>[4x]GSHMTASVPPFTVGREDPRYIELSHSDNHRFVVEPEEFFLPATPDDVVASLQKAVTEGRGVACRSGGHCGQDFVGTPRRDLVLDLHNLHAIGPAADGAGVRVGSGATVDQVQKALFRRWNAALPLGACSAVGMGGLVAG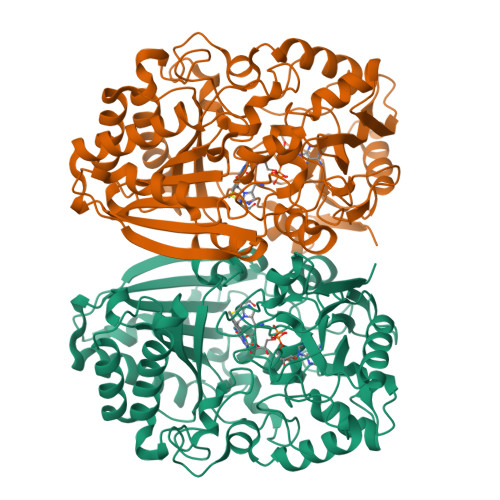GGYGPLSRQLGLVVDHLHAVEVAVVDESRTVRLVTARADDTGDLGELFWAHTGGGGGNFGVVTAYEFRSPEHLATEPVGLPRAAGRLHVQKVVFPWAMIDETSFVTVMRRFFEWHERHSEPGSPESSLFATFFVNHVSSGVLQLMVQQDADVDPEGEILARFVASLTEGTGVVGIPRGGVMSWLTGTRYMSQADCGDVMGARSASKSAYHRAAPTDEQLSVLHRHLHADHPGQASYVMFNSYGGEINRRGPSDAAVPQRDSVVKSSWFSAWQDAELDELHLGWLRGLYEEFFAGTGGVPVTGGRTDGCYINYPDADLLDPARNRSGEPWHHLYYKDNYARLRSAKRAWDPLNTFHHSMSIGL The protein that gives the process its name, Clathrin, is a triskelion composed of three heavy chains (Clathrin Heavy Chain, Chc) that provide the structural backbone of the lattice, further stabilized and regulated by three light chains (Clathrin Light Chain, Clc). The proximal domain specifically interacts with Clcs, whereas, the N-terminal domain (NTD) of Chc, which adopts a WD40 beta-propeller structure, is pivotal for interactions with various adaptor proteins (APs). To investigate the existence of binding sites present in Clathrin NTD, we crystallized the N-terminal domain of Chc with different peptides derived from adaptor proteins containing CBMs. All our structures show that each peptide binds to three different binding pockets (Clathrin, Arrestin and W-box).

Crystal structure of Chc-NTD (displayed as a grey cartoon) bound to CBMs from Ent1 (1.75 Å, red), Ent2 (1.74 Å, yellow), Ent5 (Ent5.1 LIDL motif, 2.01 Å, green), Apl2.1 (Apl2.1 LLDLF motif, 2.75 Å, blue) and Yap1801 (1.95 Å, grey). In the Clathrin box; K63 and K96 establish salt bridges with position +3 of the motif. While these interactions are consistently observed in all peptides, an exception is noted for Ent5.1, where no density for the Asp residues at positions +5 and +6 is observed. Additionally, K98 interacts with position −2 of the motif as observed in the Ent5.1, Apl2.1 and Yap1801 complexes. Concurrently, K326 forms hydrogen bonds with the peptide backbone at positions +2, +4 and +1 for the Ent5.1, Apl2.1 and Yap1801 complexes. We find that yeast epsin Ent5 has the highest affinity for clathrin, highlighting its key role in cellular trafficking. The CBM showing the highest affinity for NTD, belongs to Ent5 and is characterized by the presence of negative charges surrounding the core motif. To gain further insight into the different binding sites of Chc, we performed native mass spectrometry (native MS) experiments on Ent5.1 CBM, the strongest binder of the evaluated peptides. At experimentally suitable concentrations (up to 100 µM), we observed the appearance of Chc bound to three peptides and, although in much lower amounts, a fourth binding event was also detected. Therefore, Chc has (at least) two sets of binding sites with different binding affinities and/or Ent5.1 binds in a cooperative manner.

>GAMAMSDLPIEFTELVDLMSLGISPQFLDFRSTTFESDHFVTVRETKDGTNSVAIVDLAKGNEVTRKNMGGDSAIMHPSQMVISVRANGTIVQIFNLETKSKLKSFTLDEPVIFWRWLSETTLGFVTARSILTSNVFDGNVNAKPQLLTLRHANLNNTQIINFVANKNLDWFAVVGILQENGRIAGRIQLFSKQRNISQAIDGHVAIFTNILLEGNGSTPVQVFVTGNRNATTGAGELRIIEIDHDASLPSQYQKETTDIFFPPDATNDFPIAVQVSEKYGIIYLLTKYGFIHLYELETGTNLFVNRITAESVFTAAPYNHENGIACINKKGQVLAVEISTSQIVPYILNKLSNVALALIVATRGGLPGADDL[3x];>[9x]IPDLIDLDD>[2x]EVNLDRYQTALEEVLSWLLSAEDTLQAQGEISNDVEVVKDQFHTHEGYMMDL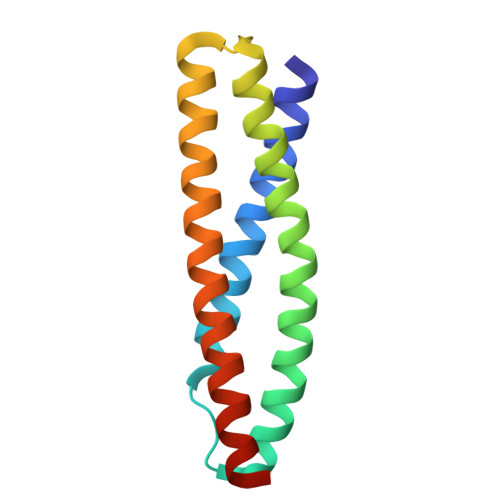TAHQGRVGNILQLGSKLIGTGKLSEDEETEVQEQMNLLNSRWECLRVASMEKQSNLHRVLMDLQNQK>[2x]MEEPEEPADSGQSLVPVYIYSPEYVSMCDSLAKIPKRASMVHSLIEAYALHKQMRIVKPKVASMEEMATFHTDAYLQHLQKVSQEGDDDHPDSIEYGLGYDCPATEGIFDYAAAIGGATITAAQCLIDGMCKVAINWSGGWHHAKKDEASGFCYLNDAVLGILRLRRKFERILYVNLDLHHGDGVEDAFSFTSKVMTVSLHKFSPGFF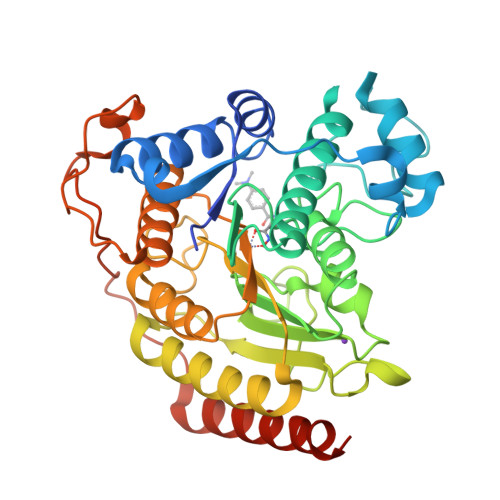PGTGDVSDVGLGKGRYYSVNVPIQDGIQDEKYYQICESVLKEVYQAFNPKAVVLQLGADTIAGDPMCSFNMTPVGIGKCLKYILQWQLATLILGGGGYNLANTARCWTYLTGVILGKTLSSEIPDHEFFTAYGPDYVLEITPSCRPDRNEPHRIQQILNYIKGNLKHVVIEGRGSHHHHHH> MGVIMNQETLIAAVEQMRKLVPALRKVPDETLYAWVEMAELFVCQKTFKDAYVKAIALYALHLAFLDGALKGEDEDLESYSRRVTSFS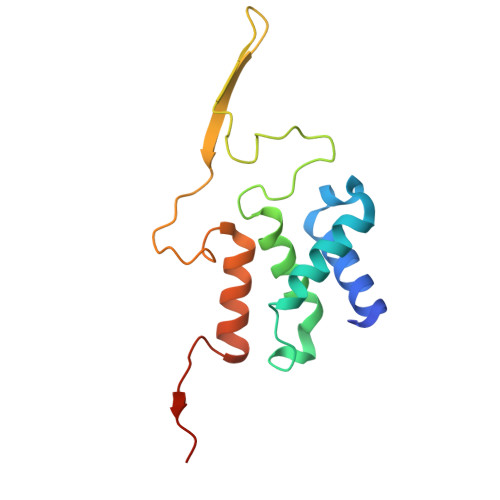LSGEFSQTFGEVTKNQSGNMMLSTPWGKMFEQLKARRRGRFALMTGLRGGCH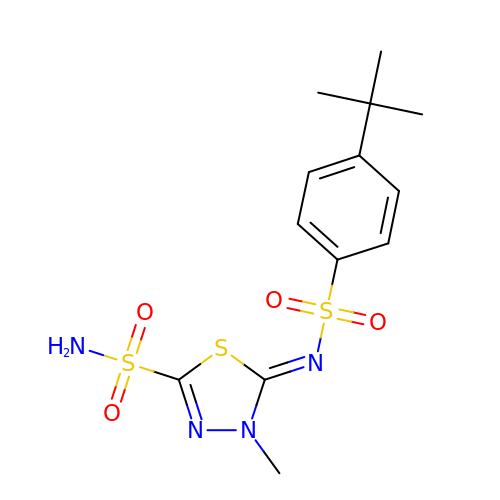(5Z)-5-{[(4-tert-butylphenyl)sulfonyl]imino}-4-methyl-4,5-dihydro-1,3,4-thiadiazole-2-sulfonamide | C13 H18 N4 O4 S3 | NSQKDLKNBCRMRT-WJDWOHSUSA-N>[2x]HPLPLPKNKHVFHSDQRLAPEIRDLYDCLYKLYAEESASEYFREPVDALRVGAWNYYSVITEPMSLRTVLDYIVQGGRYSHVEQIMNDVELIWKNCERYNG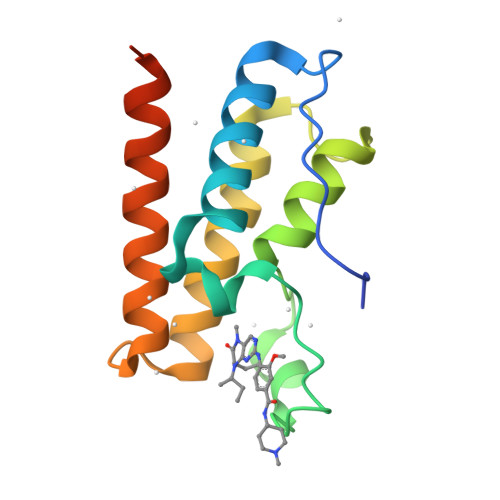AESHLAADARRCRAILEKHRERLADEQTAPAAEVD> SSSQGLLGYYFSDLNFQAPMVVTSSTTGDLSIPSSELENIPSE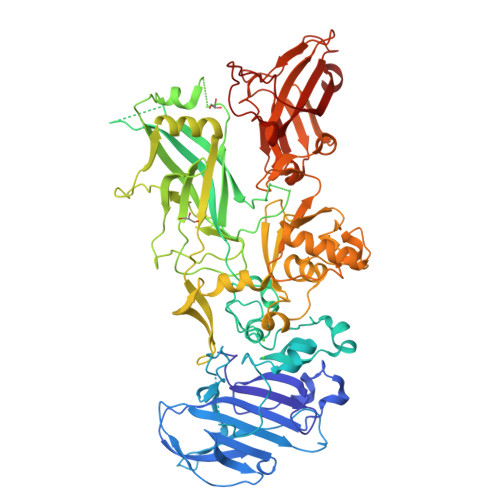NQYFQSAIWSGFIKVKKSDEYTFATSADNHVTMWVDDQEVINKASNSNKIRLEKGRLYQIKIQYQRENPTEKGLDFKLYWTDSQNKKEVISSDNLQLPELKQKSSNSRKKRSTSAGPTVPDRDNDGIPDSLEVEGYTVDVKNKRTFLSPWISNIHEKKGLTKYKSSPEKWSTASDPYSDFEKVTGRIDKNVSPEARHPLVAAYPIVHVDMENIILSKNEDQSTQNTDSQTRTISKNTSTSRTHTSEVHGNAEVHASFFDIGGSVSAGFSNSNSSTVAIDHSLSLAGERTWAETMGLNTADTARLNANIRYVNTGTAPIYNVLPTTSLVLGKNQTLATIKAKENQLSQILAPNNYYPSKNLAPIALNAQDDFSSTPITMNYNQFLELEKTKQLRLDTDQVYGNIATYNFENGRVRVDTGSNWSEVLPQIQETTARIIFNGKDLNLVERRIAAVNPSDPLETTKPDMTLKEALKIAFGFNEPNGNLQYQGKDITEFDFNFDQQTLQNIKNQLAELNATNIYEVLDKIKLNAKMNILIRDKRFHYDRNNIAVGADESVVKEAHREVINSSTEGLLLNIDKDIRKILSGYIVEIEDTEGLKEVINDRYDMLNISSLRQDGKTFIDFKKYNDKLPLYISNPNYKVNVYAVTKENTIINPSENGDTSTNGIKKILIFSKKGYEIG1-ACETYL-4-(4-{[(2S,4R)-2-(2,4-DICHLOROPHENYL)-2-(1H-IMIDAZOL-1-YLMETHYL)-1,3-DIOXOLAN-4-YL]METHOXY}PHENYL)PIPERAZINE 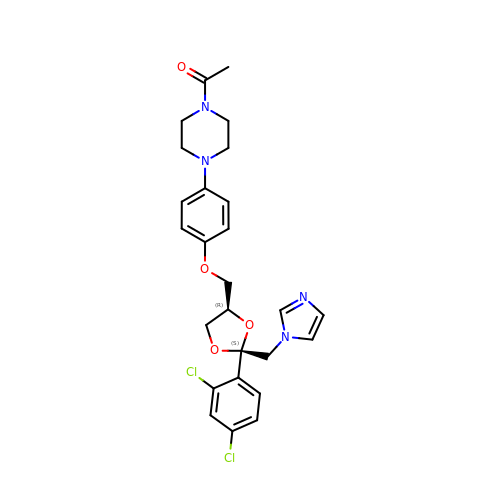| C26 H28 Cl2 N4 O4 | XMAYWYJOQHXEEK-ZEQKJWHPSA-N To neutralize chemokines, ticks secrete small cysteine-rich chemokine-binding proteins in their saliva with no homologues in mammals, termed Evasins. In contrast to the highly selective Evasin-1, its homologue Evasin-4 binds ∼20 CC-chemokines with nanomolar affinity. Among this broad range of chemokines, the chemokine CC-motif ligand 5 (CCL5, also known as RANTES) is of particular interest, because it is one of the most expressed chemokines by activated platelets and plays a prominent role in the development of atherosclerosis. Thus, Evasin-4 binds to the CCL5 monomer and causes disruption of the CCL5 dimer by shifting the monomer/dimer equilibrium toward the monomeric form of the chemokine and not by direct replacing of CCL5 from the dimer.

Here, we present the crystal structure of Evasin-4 at 1.3 Å resolution, which presents new structural features within the Evasin family members. The overall architecture of the Evasin-4 can be divided into an N- and C-terminal subdomain. Each of the N- and C-terminal subdomains consists of a three-stranded anti-parallel β-sheet core, in which the sheets are oriented orthogonally with respect to each other, forming an L-shaped structure. The 3D fold of Evasin-4 is tightly arranged by four disulfide bonds and contains a rigid protein core. Three disulfide bonds connect β-strands within a subdomain (Cys27–Cys46 connects β1 and β3, Cys63–Cys94 links β5 and β7, and Cys84–Cys103 connects β6 and β8), whereas the fourth disulfide bond (Cys42–Cys89) joins the N-terminal subdomain with the β6-strand of the C-terminal subdomain. Superposition of all six polypeptide chains of the three Evasin-4 crystal forms showed that the rigid Evasin-4 protein core is flanked by two more flexible protrusions. Residues Glu1–Glu15 are unresolved in all three crystal forms as a result of high flexibility. The crystal packing reveals a large intermolecular interface of 2,380 Å2 buried surface area common to all three Evasin-4 crystal forms. This interface involves the N-terminal region of Evasin-4 that forms an extended intermolecular antiparallel β-sheet, predominantly involving strand β1 next to strands β3 and β4 of each molecule. Thus, one can conclude that Evasin-4 is a functional monomer, whereas the observed dimer interactions in the crystal structure are a result of crystal packing.

> EVPQMTSSSAPDLEEEDDYTAYAPLTCYFTNSTLGLLAPPNCSVLCNSTTTWFNETSPNNASCLLTVDFLTQDAILQENQPYNCSVGHCDNGTCAGPPRHAQCW3,6-Bis[(3-morpholinopropionamido)] acridine | C27 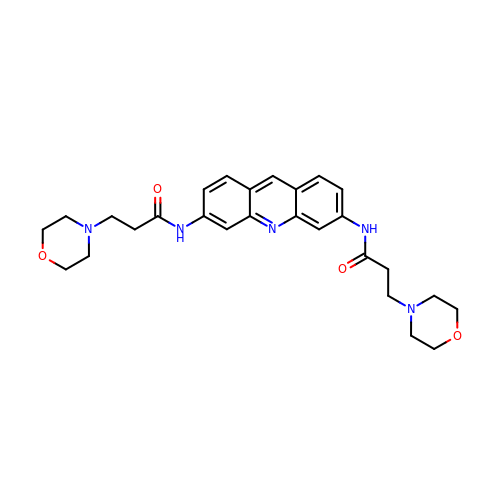H33 N5 O4 | PKCWQSROJQAQMV-UHFFFAOYSA-N> WRHIRAEGLDSSYTVLFGKAEADEIFQELEKEVEYFTGALARVQVFGKWHSVPRKQATYGD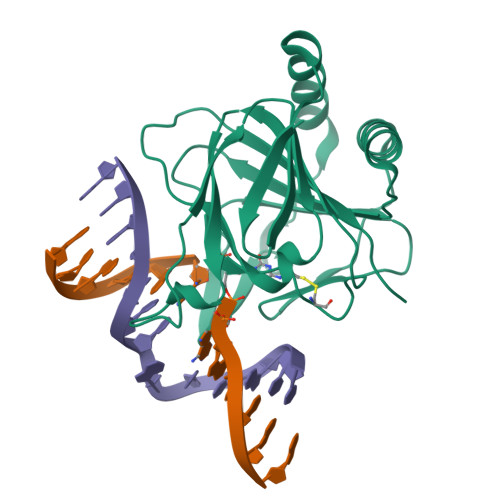AGLTYTFSGLTLSPKPWIPVLERIRDHVSGVTGQTFNFVLINRYKDGSDHIGEHRDDCRELAPGSPIASVSFGASRDFVFRHKDSRGKSPSRRVAVVRLPLAHGSLLMMNHPTNTHWYHSLPVRKKVLAPRVNLTFRKILL In a CRISPR-Cas system, Cas proteins form a complex with a small CRISPR RNA (crRNA) to detect and cleave invading nucleic acid (DNA or RNA) that has a complementary sequence to the crRNA. The Csm complex, with the RNA cleavage site located in Csm3 subunits, targets and cleaves ssRNA at 6-nucleotide intervals. In this study, we determined the cryo-EM structures of the Csm complex from Streptococcus thermophilus, with or without target ssRNA, at 3.3–3.5 Å. The results showed that the Csm complex displays a spiral-like architecture, with two spirally stacked density columns, including a single Cas10, a single Csm4, and multiple copies of Csm2 and Csm3.

We determined the near-atomic resolution structures of Csm proteins complexed with a 40 nt crRNA (from Streptococcus thermophilus), with or without 49 nt target ssRNA-bound, using cryo-EM single particle analysis. The cryo-EM micrographs and 2D class averages of both complexes display clearly a worm-like shape with mixed particle sizes. These heterogeneous particle images were classified computationally into two particle populations each yielding three-dimensional (3-D) reconstructions for the apo state (big [3.4 Å], and small [3.3 Å]) and for the target ssRNA-bound state (big [3.4 Å], and small [3.5 Å]). In total, the big maps contain 7 repeating Csm3 and 5 repeating Csm2 subunits, while the small maps contain 5 copies of Csm3 and 3 copies of Csm2. The apo and target ssRNA-bound states also correspond to DNase inactive and activated states of the complex, respectively. In our structure, an endogenous ATP molecule was observed in both the apo and target ssRNA-bound states, within the Cas10-formed binding pocket. The adenine ring of the ATP stacks against the aromatic side chain of Tyr298 in Cas10. The pentose moiety and phosphoryl atoms of the ATP molecule are in close proximity to residues His303, Lys635, Asp575/576, and Leu521 of Cas10. The structural comparison between the apo and target ssRNA-bound states of the Csm complex revealed no substantial structural difference between the two structures. However, we do notice a small shift in the Csm2 proteins in the target ssRNA-bound state compared to the apo state. The shift is more pronounced in Csm2a (~1.2 Å) than in Csm2b (~0.9 Å) or Csm2c (negligible).

>[3x]MAILTDENYVDKAERAISLLEKDNKGNYLLTTSQIRKLLSLCSSLYDRSKERKFDELINDVSYLRVQFVYQAGREIAVKDLIEKAQILEALKEIKDRETLQRFCRYMEALVAYFKFYGGKD;>[5x]MTFAKIKFSAQIRLETGLHIGGSDAFAAIGAIDSPVIKDPITNIPIIPGSSLKGKMRTLLAKVYNEKVAEKPSDDSDILSRLFGNSKDKRFKMGRLIFRDAFLSNADELDSLGVRSYTEVKFENTIDRITAEANPRQIERAIRNSTFDFELIYEITDENENQVEEDFKVIRDGLKLLELDYLGGSGSRGYGKVAFEKLKATTVFGNYDVKTLNELLTAEV;> MTYKLYIMTFQNAHFGSGTLDSSKLTFSADRIFSALVLESLKMGKLDAFLAEANQDKFTLTDAFPFQFGPFLPKPIGYPKHDQIDQSVDVKEVRRQAKLSKKLQFLALENVDDYLNGELFENEEHAVIDTVTKNQPHKDGNLYQVATTRFSNDTSLYVIANESDLLNELMSSLQYSGLGGKRSSGFGRFELDIQNIPLELSDRLTKNHSDKVMSLTTALPVDADLEEAMEDGHYLLTKSSGFAFSHATNENYRKQDLYKFASGSTFSKTFEGQIVDVRPLDFPHAVLNYAKPLFFKLEV;> MKKEKIDLFYGALLHDIGKVIQRATGERKKHALVGADWFDEIADNQVISDQIRYHMANYQSDKLGNDHLAYITYIADNIASGVDRRQSNEESDEDASAKIWDTYTNQADIFNVFGAQTDKRYFKPTVLNLKSKPNFASATYEPFSKGDYAAIATRIKNELAEFEFNQAQIDSLLNLFEAILSFVPSSTNSKEIADISLAEHSRLTAAFALAIYDYLEDKGRHNYKEDLFTKASAFYEEEAFLLASFDLSGIQDFIYNIATSGAAKQLKARSLYLDFMSEYIADSLLDKLGLNRANLLYVGGGHAYFVLANTEKTVETLVQFEKDFNQFLLANFQTRLYVAFGWGSFAAKDIMSELNSPESYRQIYQKASRMISEKKISRYDYRTLMLLNRGGKSSERECEICHSVENLVSYHDQKVCDICRGLYQFSKEIAHDHFIITENEGLPIGPNACLKGVAFEKLSQESFSRVYVKNDYKAGTIKATHVFVGDYQCDEIHKYAALSKNEDGLGIKRLAVVRLDVDDLGAAFMAGFSRQGNGQYSTLSRSATFSRSMSLFFKVYINQFASDKKLSIIYAGGDDVFAIGSWQDIIAFTVELRQNFIKWTNGKLTLSAGIGLFADKTPISLMAHQTGELEEAAKGNEKDSISLFSSDYTFKFDRFITNVYDDKLEQIRYFFNHQDERGKNFIYKLIELLRNYESEEKMNVARLAYYLTRLEELTDKDERDKFKQFKKLFFKWYTNNESDRKEAELALLLYVYEIRKD1,3-dichloropropane 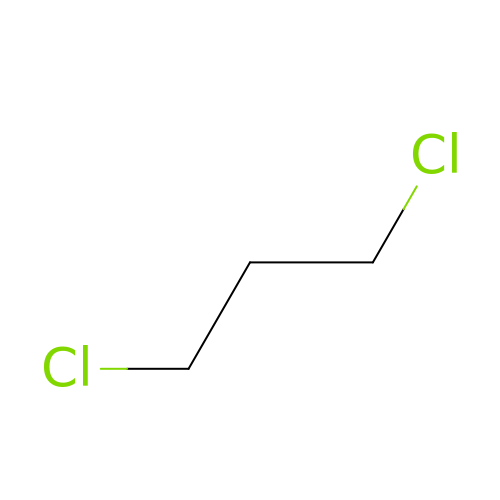| C3 H6 Cl2 | YHRUOJUYPBUZOS-UHFFFAOYSA-N> MISQSRYIRIISGVGAAAPVAGRKLILRVMTTNNVIPPGIVIEFDNANAVLSYFGAQSEEYQRAAAYFKFISKSVNSPSSISFARWVNTAIAPMVVGDNLPKTIADFAGFSAGVLTIMVGAAEQNITAIDTSAATSMDNVASIIQTEIRKNADPQLAQATVTWNQNTNQFTLVGATIGTGVLAVAKSADPQDMSTALGWSTSNVVNVAGQSADLPDAAVAKSTNVSNNFGSFLFAGAPLDNDQIKAV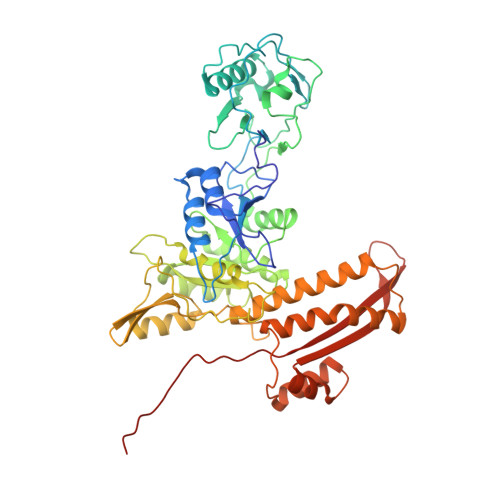SAWNAAQNNQFIYTVATSLANLGTLFTLVNGNAGTALNVLSATAANDFVEQCPSEILAATNYDEPGASQNYMYYQFPGRNITVSDDTVANTVDKSRGNYIGVTQANGQQLAFYQRGILCGGPTDAVDMNVYANEIWLKSAIAQALLDLFLNVNAVPASSTGEAMTLAVLQPVLDKATANGTFTYGKEISAVQQQYITQVTGDRRAWRQVQTLGYWINITFSSYTNSNTGLTEWKANYTLIYSKGDAIRFVEGSDVMI>MMSETAP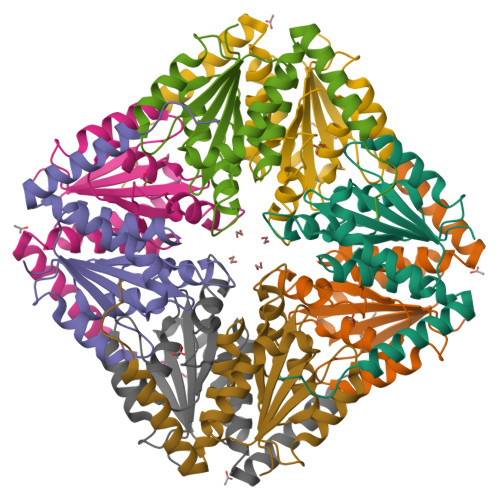LPSASSALEDKAASAPVVGIIMGSQSDWETMRHADALLTELEIPHETLIVNAHRTPDRLADYARTAAERGLNVIIAGAGGAAHLPGMCAAWTRLPVLGVPVESRALKGMDSLLSIVQMPGGVPVGTLAIGASGAKNAALLAASILALYNPALAARLETWRALQTASVPNSPITEDK[2x]>MENDPNLFVALYDFVASGDNTLSITKGEKLRVLGYNHNGEWCEAQTKNGQGWVPSQYITPVNS[2x];>XAPSYSPPPP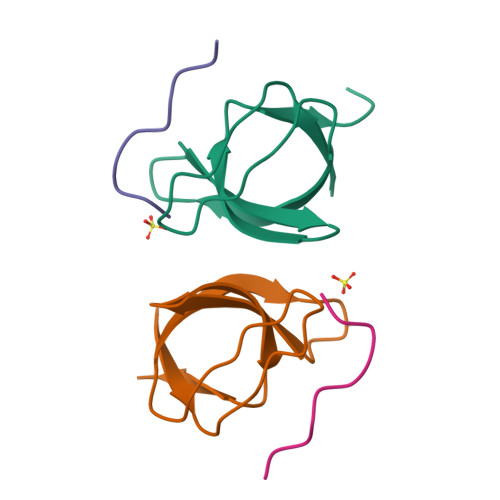P[2x]> GASGSDFPVISPFTFPTNVRLGEQVRVFCTVRRGNPPFSFAWFKEGEKLITGQHIEVENTDKYTSKLGILNVSTLDIGNYTCE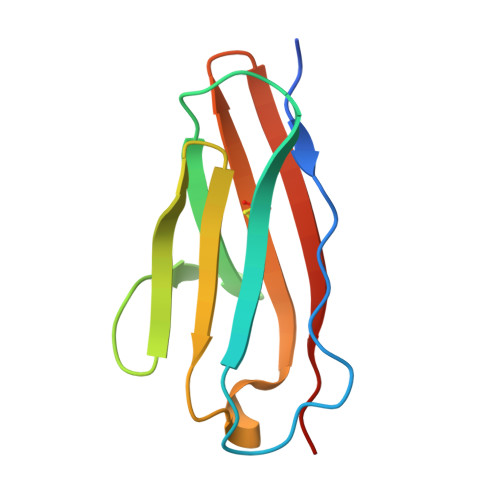ITNQDGKDSATSRLIVEAP> MGAFLDKPKMEKHNAQGQGNGLRYGLSSMQGWRVEMEDAHTAVIGL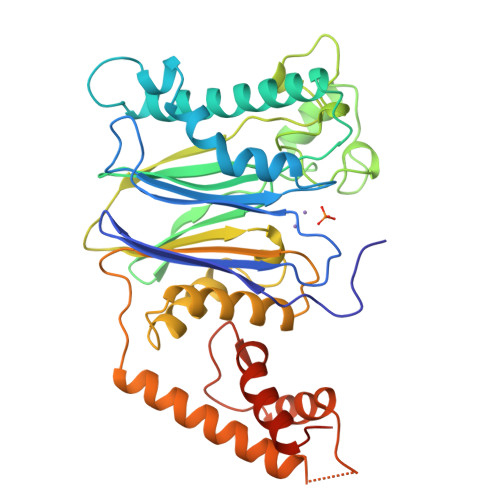PSGLESWSFFAVYDGHAGSQVAKYCCEHLLDHITNNQDFKGSAGAPSVENVKNGIRTGFLEIDEHMRVMSEKKHGADRSGSTAVGVLISPQHTYFINCGDSRGLLCRNRKVHFFTQDHKPSNPLEKERIQNAGGSVMIQRVNGSLAVSRALGDFDYKCVHGKGPTEQLVSPEPEVHDIERSEEDDQFIILACDGIWDVMGNEELCDFVRSRLEVTDDLEKVCNEVVDTCLYKGSRDNMSVILICFPNAPKVSPEAVKKEAELDKYLECRVEEIIKKQGEGVPDLVHVMRTLASENIPSLPPGGELASKRNVIEAVYNRLNPYKNDDTDSTSTDDMW> GPLG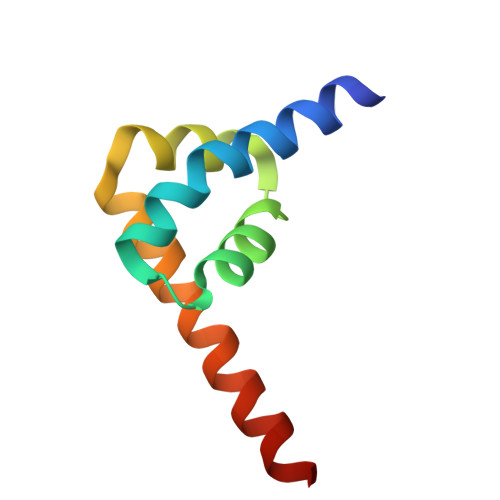SQEQKQMLGERLFPLIQAMHPTLAGKITGMLLEIDNSELLHMLESPESLRSKVDEAVAVLQAHQAKEAAQKA>SNAMILGDSEQKRRKALKKVLDAVEEHGGTTILSTGITGDDARIARAAVAGGARLLEPNHPAVALARGHKGVITMHAAEQVRHEIPLDEMLKVTQGVRNVVGEDIYITVGVPGGFTEILPL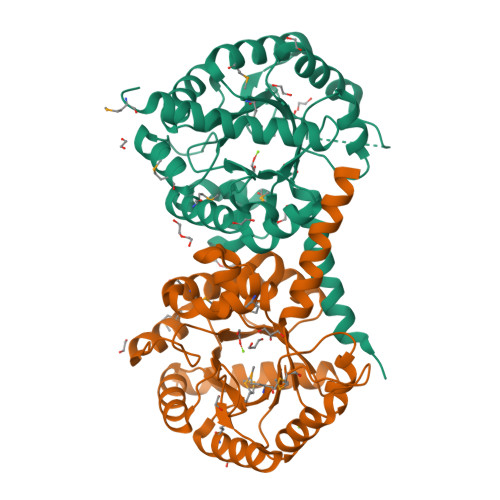ELKEEDFFKIAMSGADGVHIHKSTLEDLKDVVKYAHKYGLLVDAYIGHPDDLHTFGISARTPEEVAEAAKEMEKIGVDMIGLMTGMSYEGTAAGEIHPVIKERLSALVSSVKVPTLAEGGINDTNYVAFKDTGVNILVIGTSIDNVVSEAATNVVKKFLSLKKQA[2x]> FVVEKNNLKVTSPDSIKGIYECAIGNFGVPQYGGTLVGTVVYPKSNQKACKSYSDFDISFKSKPGRLPTFVLIDRGDCYFTLKAWIAQQAGAAAILVADSKAEPLITMDTPEEDKSDADYLQNITIPSALITKTLGDSIKSALSGGDMVNMKLDWTESVPHPDERVEYELWTNSNDECGKKCDTQIEFLKNFKGAAQILEKGGHTQFTPHYITWYCPEAFTLSKQCKSQCINHGRYCAPDPEQD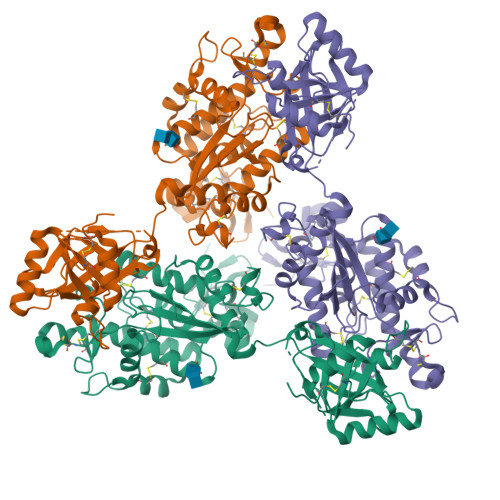FTKGYDGKDVVVQNLRQACVYRVMNDTGKPWVWWDYVTDFAIRCPMKEKKYTKECADGIIKSLGIDLKKVDKCIGDPEADVENPVLKAEQESQIGKGSRGDVTILPTLVVNNRQYRGKLEKGAVLKAMCSGFQESTEPAICLTEDLETNECLENNGGCWQDKAANITACRDTFRGRLCECPTVQGVKFVGDGYTHCKASGALHCGINNGGCWRESRGGFTYSACVDDHSKDCKCPLGFKGDGVKNCEDVDECKEKTVCQCPECKCKNTWGSYECSCSNGLLYMREHDTCIGSGKVGTTKLSWSFLWILIIGVGVAGLS>[2x]GEIRPTIGQQMETGDQRFGDLVF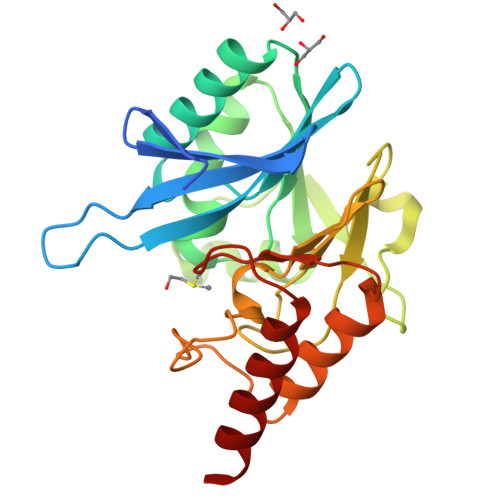RQLAPNVWQHTSYLDMPGFGAVASNGLIVRDGGRVLVVDTAWTDDQTAQILNWIKQEINLPVALAVVTHAHQDKMGGMDALHAAGIATYANALSNQLAPQEGMVAAQHSLTFAANGWVEPATAPNFGPLKVFYPGPGHTSDNITVGIDGTDIAFGGCLIKDSKAKSLGNLGDADTEHYAASARAFGAAFPKASMIVMSHSAPDSRAAITHTARMADKLRKL>[4x]MYQKFKGGDLMIHGGDIYTEGVFKGRELLDYSSNINPLGIPKSFLNNIDEGIKNLGVYPDVNYRRLNKSIENYLKLKDIGIVLGNGASEIIELSISLFEKILIIVPSYAEYEINAKKHGVSVVFSYLDENMCIDYEDIISKIDDVDSVIIGNPNNPNGGLINKEKFIHVLKLAEEKKKTIIIDEAFIEFTGDPSSSFVGEIKNYSCLFIIRAMTKFFAMPGIRFGYG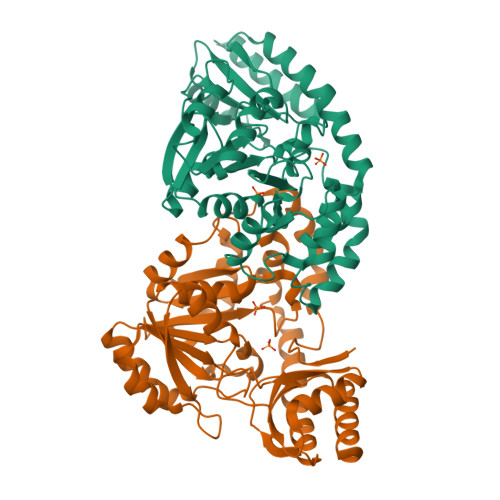ITNNKEIAAKIKAKQNPWNINCFAEMAAINCLKDTNYIEESLLWIKKERKRFIEELNKIGFIKRVFSPHANFVLCRLENISGEKLYDSLLKEDIVIRRCCNFIGLDDSFVRFAIKDEKKNTKFLRALKGVENNL>HMCLVCSDEASGCHYGVLTCGSCKVFFKRAVEG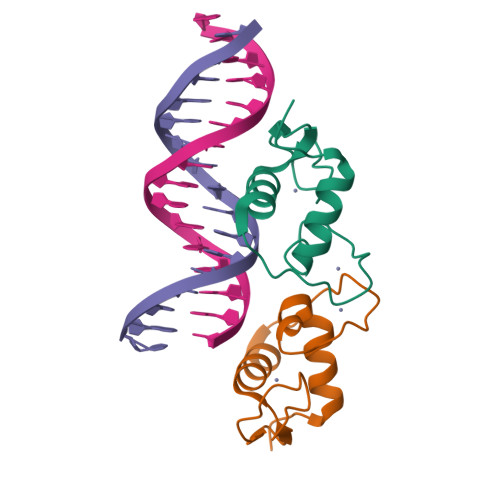QHNYLCAGRNDCIIDKIRRKNCPACRYRKCLQAGMNLEA[2x]> MQKVGIYPGTFDPVTNGHIDIIHRSSELFEKLIVAVAHSSAKNPM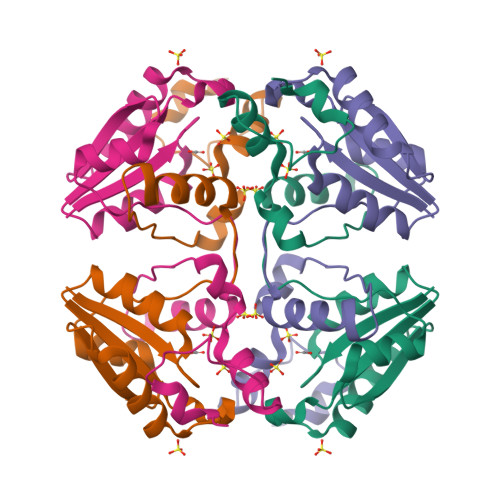FSLDERLKMIQLATKSFKNVECVAFEGLLAYLAKEYHCKVLVRGLRVVSDFEYELQMGYANKSLNHELETLYFMPTLQNAFISSSIVRSIIAHKGDASHLVPKEIYPLISKA>MAHHHHHHSSGLEVLFQGPMNESVKEIPDVLKSQSGFNSLTDISHSSFNEFRQQVSEHLSWSETHDLYHDAQQAQKDNRLYEARILKRANPQLQNAVHLAILAPNAELIGYNNQFSGRASQYVAPGTVSSMFSPAAYLTELYREARNLHASDSVYYLDTRRPDLKSMALSQQNMDIELSTLSLSNELLLESIKTESKLENYTKVMEMLSTFRPSGATPYHDAYENVREVIQLQDPGLEQLNASPAIAGLMHQASLLGINASISPELFNILTEEITEGNAEELYKKNFGNIEPASLAMPEYLKRYYNLSDEELSQFIGKASNFGQQEYSNNQLITPVVNSSDGTVKVYRITREYTTNAYQMDVELFPFGGENYRLDYKFKNFYNASYLSIKLNDKRELVRTEGAPQVNIEYSANITLNTADISQPFEIGLTRVLPSGSWAYAAAKFTVEEYNQYSFLLKLNKAIRLSRATELSPTILEGIVRSVNLQLDINTDVLGKVFLTKYYMQRYAIHAETALILCNAPISQRSYDNQPSQFDRLFNTPLLNGQYFSTGDEEIDLNSGSTGDWRKTILKRAFNIDDVSLFRLLKITDHDNKDGKIKNNLKNLSNLYIGKLLADIHQLTIDELDLLLIAVGEGKTNLSAISDKQLATLIRKLNTITSWLHTQKWSVFQLFIMTSTSYNKTLTPEIKNLLDTVYHGLQGFDKDKADLLHVMAPYIAATLQLSSENVAHSVLLWADKLQPGDGAMTAEKFWDWLNTKYTPGSSEAVETQEHIVQYCQALAQLEMVYHSTGINENAFRLFVTKPEMFGAATGAAPAHDALSLIMLTRFADWVNALGEKASSVLAAFEANSLTAEQLADAMNLDANLLLQASIQAQNHQHLPPVTPENAFSSWTSINTILQWVNVAQQLNVAPQGVSALVGLDYIQSMKETPTYAQWENAAGVLTAGLNSQQANTLHAFLDESRSAALSTYYIRQVAKAAAAIKSRDDLYQYLLIDNQVSAAIKTTRIAEAIASIQLYVNRALENVEENANSGVISRQFFIDWDKYNKRYSTWAGVSQLVYYPENYIDPTMRIGQTKMMDALLQSVSQSQLNADTVEDAFMSYLTSFEQVANLKVISAYHDNINNDQGLTYFIGLSETDAGEYYWRSVDHSKFNDGKFAANAWSEWHKIDCPINPYKSTIRPVIYKSRLYLLWLEQKEITKQTGNSKDGYQTETDYRYELKLAHIRYDGTWNTPITFDVNKKISELKLEKNRAPGLYCAGYQGEDTLLVMFYNQQDTLDSYKNASMQGLYIFADMASKDMCPEQSNVYRDNSYQQFDTNNVRRVNNRYAEDYEIPSSVSSRKDYGWGDYYLSMVYNGDIPTINYKAASSDLKIYISPKLRIIHNGYEGQKRNQCNLMNKYGKLGDKFIVYTSLGVNPNNSSNKLMFYPVYQYSGNTSGLNQGRLLFHRDTTYPSKVEAWIPGAKRSLTNQNAAIGDDYATDSLNKPDDLKQYIFMTDSKGTATDVSGPVEINTAISPAKVQIIVKAGGKEQTFTADKDVSIQPSPSFDEMNYQFNALEIDGSGLNFINNSASIDVTFTAFAEDGRKLGYESFSIPVTLKVSTDNALTLHHNENGAQYMQWQSYRTRLNTLFARQLVARATTGIDTILSMETQNIQEPQLGKGFYATFVIPPYNLSTHGDERWFKLYIKHVVDNNSHIIYSGQLTDTNINITLFIPLDDVPLNQDYHAKVYMTFKKSPSDGTWWGPHFVRDDKGIVTINPKSILTHFESVNVLNNISSEPMDFSGANSLYFWELFYYTPMLVAQRLLHEQNFDEANRWLKYVWSPSGYIVHGQIQNYQWNVRPLLEDTSWNSDPLDSVDPDAVAQHDPMHYKVSTFMRTLDLLIARGDHAYRQLERDTLNEAKMWYMQALHLLGDKPYLPLSTTWSDPRLDRAADITTQNAHDSAIVALRQNIPTPAPLSLRSANTLTDLFLPQINEVMMNYWQTLAQRVYNLRHNLSIDGQPLYLPIYATPADPKALLSAAVATSQGGGKLPESFMSLWRFPHMLENARGMVSQLTQFGSTLQNIIERQDAEALNALLQNQAAELILTNLSIQDKTIEELDAEKTVLEKSKAGAQSRFDSYGKLYDENINAGENQAMTLRASAAGLTTAVQASRLAGAAADLVPNIFGFAGGGSRWGAIAEATGYVMEFSANVMNTEADKISQSETYRRRRQEWEIQRNNAEAELKQIDAQLKSLAVRREAAVLQKTSLKTQQEQTQSQLAFLQRKFSNQALYNWLRGRLAAIYFQFYDLAVARCLMAEQAYRWELNDDSARFIKPGAWQGTYAGLLAGETLM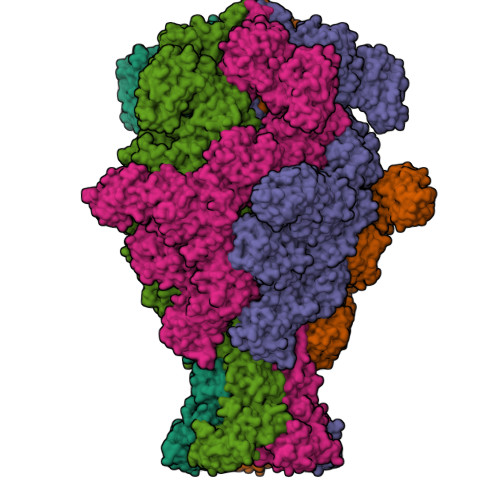LSLAQMEDAHLKRDKRALEVERTVSLAEVYAGLPKDNGPFSLAQEIDKLVSQGSGSAGSGNNNLAFGAGTDTKTSLQASVSFADLKIREDYPASLGKIRRIKQISVTLPALLGPYQDVQAILSYGDKAGLANGCEALAVSHGMNDSGQFQLDFNDGKFLPFEGIAIDQGTLTLSFPNASMPEKGKQATMLKTLNDIILHIRYTIK[5x]>[2x]SELRDRQAIFETLVAKGRELLACDRVIVYAFDDNYVGTVVAESVAEGWPQARDQVIEDPCFREHWV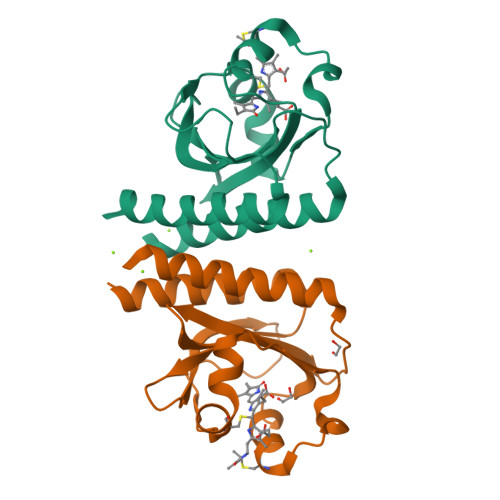EAYRQGRIQATTDIFKAGLTECHLNQLRPLKVRANLVVPMVIDDQLFGLLIAHQASEPRQWQEIEIDQFSELASTGSLVLERLH>[2x]MKMTSIQQRAELHRQIWQIANDVRGSVDGWDFKQYVLGALFYRFISENFSSYIEAGDDSICYAKLDDSVITDDIKDDAIKTKGYFIYPSQLFCNVAAKANTNDRLNADLNSIFVAIESSAYGYPSEADIKGLFADFDTTSNRLGNTVKDKNARLAAVLKGVEGLKLGDFNEHQIDLFGDAYEFLISNYAANAGKSGGEFFTPQHVSKLIAQLAMHGQTHVNKIYDPAAGSGSLLLQAKKQFDNHIIEEGFFGQEINHTTYNLARMNMFLHNINYDKFDIKLGNTLTEPHFRDEKPFDAIVSNPPYSVKWIGSDDPTLINDERFAPAGVLAPKSKADFAFVLHALNYLSAKGRAAIVCFPGIFYRGGAEQKIRQYLVDNNYVETVISLAPNLFFGTTIAVNILVLSKHKTDTNVQFIDASELFKKETNNNILTDAH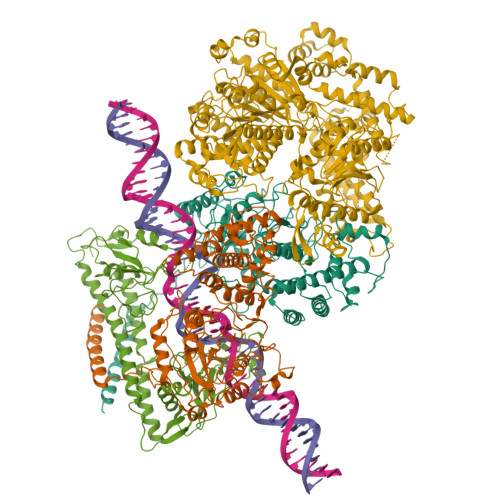IEQIMQVFASKEDVAHLAKSVAFETVVANDYNLSVSSYVEAKDNREIIDIAELNAELKTTVSKIDQLRKDIDAIVAEIEGCEVQK;> MSEMSYLEKLLDGVEVEWLPLGEITKYEQPTKYLVKAKDYHDTYTIPVLTAGKTFILGYTNETHGIYQASKAPVIIFDDFTTANKWVDFDFKAKSSAMKMVTSCDDNKTLLKYVYYWLNTLPSEFAEGDHKRQWISNYSQKKIPIPCPDNPEKSLAIQSEIVRILDKFTALTAELTAELNMRKKQYNYYRDQLLSFKEGEVEWKTLGEIGKWYGGGTPSKNKIEFWENGSIPWISPKDMGRTLVDSSEDYITEEAVLHSSTKLIPANSIAIVVRSSILDKVLPSALIKVPATLNQDMKAVIPHENILVKYIYHMIGSRGSDILRAAKKTGGSVASIDSKKLFSFKIPVPNINEQQRIVEILDKFDTLTNSITEGLPREIELRQKQYEYYRDLLFSFPKPETVSN;> MTHQTHTIAESNNFIVLDKYIKAEPTGDSYQSESDLERELIQDLRNQGYEFISVKSQSAMLANVREQLQNLNGVVFNDSEWRRFTEQYLDNPSDGILDKTRKIHIDYICDFIFDDERLENIYLIDKKNLMRNKVQIIQQFEQAGSHANRYDVTILVNGLPLVQIELKKRGVAIREAFNQIHRYSKESFNSENSLFKYLQLFVISNGTDTRYFANTTKRDKNSFDFTMNWAKSDNTLIKDLKDFTATCFQKHTLLNVLVNYSVFDSSQTLLVMRPYQIAATERILWKIKSSFTAKNWSKPESGGYIWHTTGSGKTLTSFKAARLATELDFIDKVFFVVDRKDLDYQTMKEYQRFSPDSVNGSENTAGLKRNLDKDDNKIIVTTIQKLNNLMKAESDLPVYNQQVVFIFDECHRSQFGEAQKNLKKKFKRYYQFGFTGTPIFPENALGSETTASVFGRELHSYVITDAIRDEKVLKFKVDYNDVRPQFKSLETETDEKKLSAAENQQAFLHPMRIQEITQYILNNFRQKTHRTFPGSKGFNAMLAVSSVDAAKAYYATFKRLQEEAANKSATYKPLRIATIFSFAANEEQNAIGEISDETFDTSAMDSSAKEFLDAAIREYNSHFKTNFSTDSNGFQNYYRDLAQRVKNQDIDLLIVVGMFLTGFDAPTLNTLFVDKNLRYHGLMQAFSRTNRIYDATKTFGNIVTFRDLERSTIDAITLFGDKNTKNVVLEKSYTEYMEGFTDAATGEAKRGFMTVVSELEQRFPDPTSIESEKEKKDFVKLFGEYLRAENILQNYDEFATLKALQQIDLSDPVAVEKFKAEHYVDDEKFAELQTIRLPADRKIQDYRSAYNDIRDWQRREKEAEKKEKSTTDWDDVVFEVDLLKSQEINLDYILGLIFEHNRQNKGKGEMIEEVKRLIRSSLGNRAKEGLVVDFIQQTNLDDLPDKASIIDAFFTFAQREQQREAEALIKEENLNEDAAKRYIRTSLKREYATENGTELNETLPKLSPLNPQYKTKKQAVFQKIVSFIEKFKGVGGKI>MLDGAEASNGVSKQTVGGVHVTPEMLESVQIPLEADKVGMTPAEKSKLVNAATAVYIDMAVEEMRSRGLAPKADYRVHWWKVMQDFVDSGEGQRVLQETSLTNQELERVIAKLGIEGEVIARMGPEIVNILTGKTHALAHIMRDDLLFRVYLSDEGRRANRYMAEYARLLTSQRRDIRILEIGAGTGGTTSEVLNLCSPNGESFCAEYMYTDLSPGFFNAAKTTLKKWESHLAFQVLNIEDDPAGQGFKEHTYDLIIAANVIHATARLTNTLSNVHKL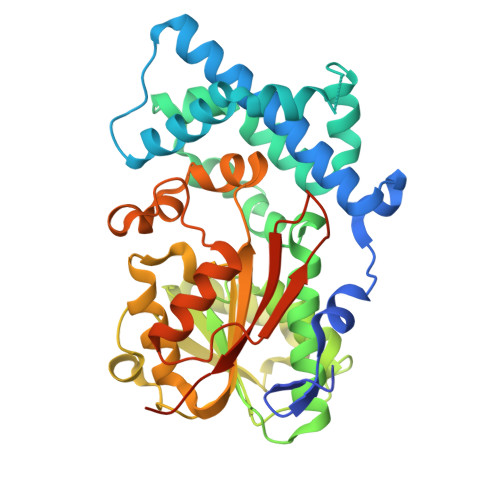LKPGGVFGLVELTRLTPFYNLTFGSLSGWWAGVDEGRTESPLQSPQQWNSLLKQTGFSGVDLAAYDLPGPERHSCLLLSTALSNSVTTNGHGHHHHHHHH[3x]>RTRRPGEPPLDLGSIPWLGYALDFGKDAASFLTRMKEKHGDIFTILVGGRYVTVLLDPHSYDAVVWEPRTRLDFHAYAIFLMERIFDVQLPHYSPSDEKARMKLTLLHRELQALTEAMYTNLHAVLLGDATEAGSGWHEMGLLDFSYSFLLRAGYLTLYGIEALPRTHESQAQDRVHSADVFHTFRQLDRLLPKLARGSLSVGDKDHMCSVKSRLWKLLSPARLARRAHRSKWLESYLLHLEEMGVSEEMQARALVL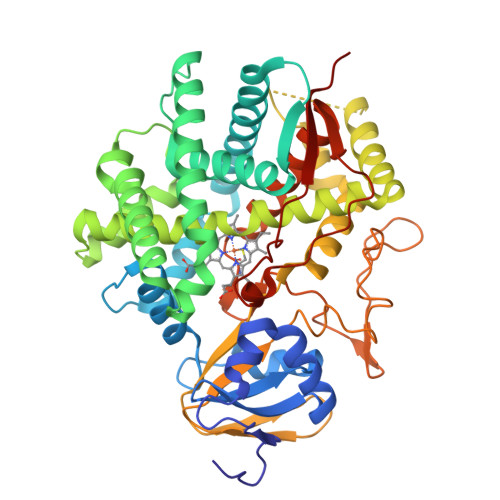QLWATQGNMGPAAFWLLLFLLKNPEALAAVRGELESILWQAEQPVSQTTTLPQKVLDSTPVLDSVLSESLRLTAAPFITREVVVDLAMPMADGREFNLRRGDRLLLFPFLSPQRDPEIYTDPEVFKYNRFLNPDGSEKKDFYKDGKRLKNYNMPWGAGHNHCLGRSYAVNSIKQFVFLVLVHLDLELINADVEIPEFDLSRYGFGLMQPEHDVPVRYRIRPHHHH[2x]> GSHMEQLKHCNGILKELLSKKHAAYAWP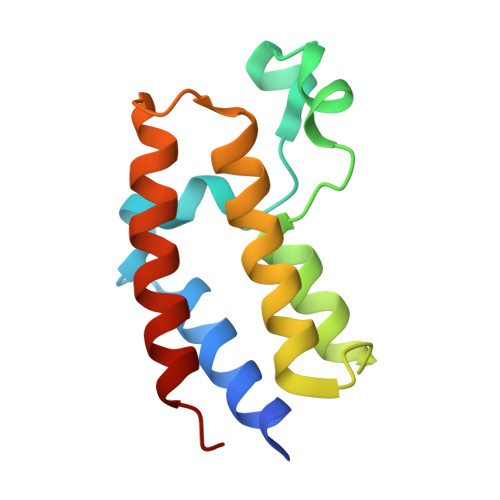FYKPVDASALGLHDYHDIIKHPMDLSTVKRKMENRDYRDAQEFAADVRLMFSNCYKYNPPDHDVVAMARKLQDVFEFRYAKMPD> ERVPEGSIRVAIASNNGEQLDGHFGSCLRFLVYQVSAKDASLVDIRSTLDVALAEDKNAWRVEQIQDCQVLYVVSIGGPAAAKVVRAGIHPLKKPKGCAAQEAIAELQTVMAG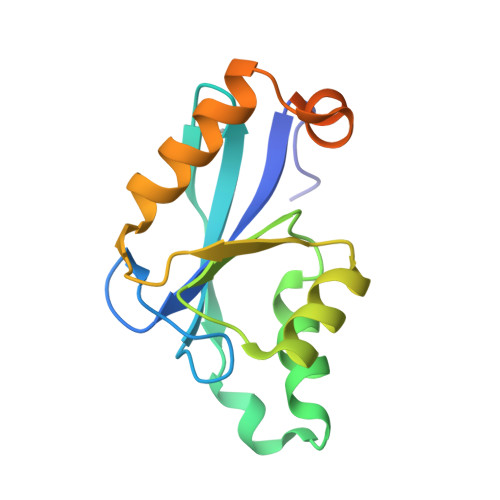SPPPWLAKLVGVSAEERVRFSVSDDEDEAARA> MKRRWKKNFIAVSAANRFKKISSSGALENLYFQGEMAKTLKDLQGWEIITTDEQGNIIDGGQKRLRRRGAKTEHYLKRSSDGIKLGRGDSVVMHNEAAGTYSVYMIQELRLNTLNNVVELWALTYLRWFEVNPLAHYRQFNPDANILNRPLNYYNKLFSETANKNELYLTAELAELQLFNFIRVANVMDGSKWEVLKGNVDPERDFTVRYICEPTGEKFVDINIEDVKAYIKKVEPREAQEYLKDLTLPSKKKEIKRGPQKKDKATQTAQISDAETRATDITDNEDGNEDESSDYESPSDIDVSEDMDSGEISADELEEEEDEEEDEDEEEKEARHTNSPRKRGRKIKLGKDDIDASVQPPPKKRGRKPKDPSKPRQMLLISSCRANNTPVIRKFTKKNVARAKKKYTPFSKRFKSIAAIPDLTSLPEFYGNSSELMASRFENKLKTTQKHQIVETIFSKVKKQLNSSYVKEEILKSANFQDYLPARENEFASIYLSAYSAIESDSATTIYVAGTPGVGKTLTVREVVKELLSSSAQREIPDFLYVEINGLKMVKPTDCYETLWNKVSGERLTWAASMESLEFYFKRVPKNKKKTIVVLLDELDAMVTKSQDIMYNFFNWTTYENAKLIVIAVANTMDLPERQLGNKITSRIGFTRIMFTGYTHEELKNIIDLRLKGLNDSFFYVDTKTGNAILIDAAGNDTTVKQTLPEDVRKVRLRMSADAIEIASRKVASVSGDARRALKVCKRAAEIAEKHYMAKHGYGYDGKTVIEDENEEQIYDDEDKDLIESNKAKDDNDDDDDNDGVQTVHITHVMKALNETLNSHVITFMTRLSFTAKLFIYALLNLMKKNGSQEQELGDIVDEIKLLIE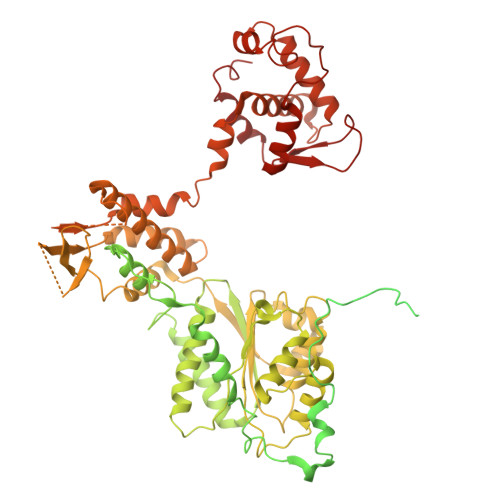VNGSNKFVMEIAKTLFQQGSDNISEQLRIISWDFVLNQLLDAGILFKQTMKNDRICCVKLNISVEEAKRAMNEDETLRNL> AQHITPVSEKKVDDKITLYKTTATSDSDKLKISQILTFNFIKDKSYDKDTLILKAAGNIYSGYTKPNPKDTISSQFYWGSKYNISINSDSNDSVNVVDYAPKNQNEEFQVQQTVGYSYGGDINISNGLSGGGNGSKSFSETINYKQESYRTSLDKRTNFKKIGWDVEAHKIMNNGWGPYGRDSYHSTYGNEMFLGSRQSNLNAGQNFLEYHKMPVLSRGNFNPEFIGVLSRKQNAAKKSKITVTYQREMDRYTNFWNQLHWIGNNYKDENRATHTSIYEVDWENHTVKLIDTQSKEKNPMS;>DNNIENIGDGAEVVKRTEDTSSDKWGVTQNIQFDFVKDKKYNKD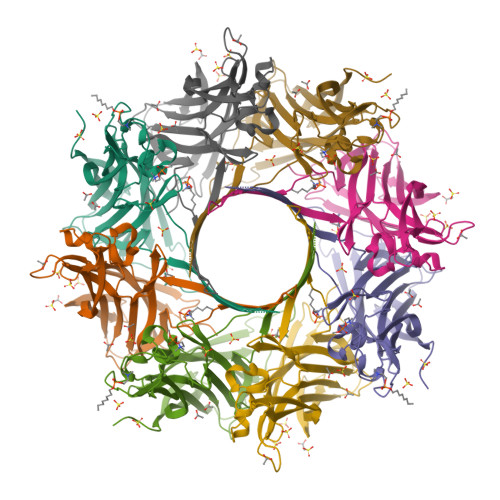ALILKMQGFINSKTTYYNYKNTDHIKAMRWPFQYNIGLKTNDPNVDLINYLPKNKIDSVNVSQTLGYNIGGNFNSGPSTGGNGSFNYSKTISYNQQNYISEVERQNSKSVQWGIKANSFITSLGKMSGHDPNLFVGYKPYSQNPRDYFVPDNELPPLVHSGFNPSFIATVSHEKGSGDTSEFEITYGRNMDVTHATRRTTHYGNSYLEGSRIHNAFVNRNYTVKYEVNWKTHEIKVKGHN[2x]> SNADTIKVGVIGTMSGPYALFGQNFKMGIDAWVAEHGNKVGGHTVEFVYRDEVSPNPAQSKALAQELIVKEKVQYIAGLYFTPNAMAVAPLLQEAKVPMVVLNAATSSITEKSPYIVRTSFTMFQNTVPAAKVAKQKGAKKVAIAVSDYGPGIDAETAFKKTFEAEGGSVVEAVRMPLATTDFGPIMQRIKDSGADMIFTFLPAGPPTLGFVKAYIDNGLKAAGVKLMSTGDVVTEPDLPNIGDSGIGILSTYHYAVSHDSPENKAFLALLQKGGAKLGDVTMTSVA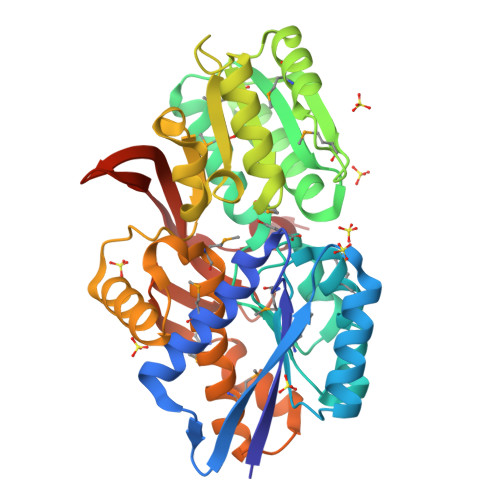AYDGARLIYKMIEATGGKQDPEKAIAAVKDMKWTSPRGPVSIDPTTRHITQSVYLREVEKQDGKLINKEIETFKDQPDWGLVKQ>[4x]MGSTGNAEIQIIPTHSSDEEANLFAMQLASAAVLPMALKAA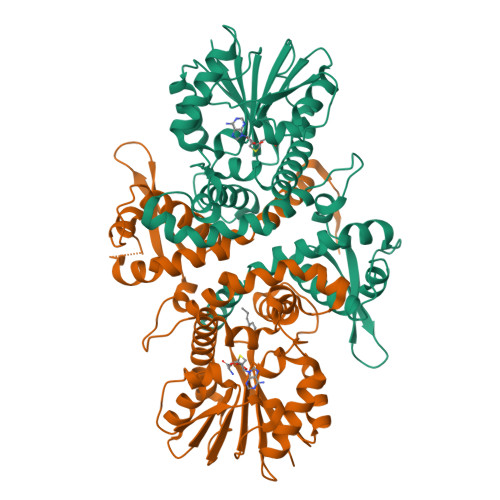IELDVLEIMAKSVPPSGYISPAEIAAQLPTTNPEAPVMLDRVLRLLASYSVVTYTLRELPSGKVERLYGLAPVCKFLTKNEDGVSLAPFLLLATDKVLLEPWFYLKDAILEGGIPFNKAYGMNIFDYHGTDHRINKVFNKGMSSNSTITMKKILEMYNGFEGLTTIVDVGGGTGAVASMIVAKYPSINAINFDLPHVIQDAPAFSGVEHLGGDMFDGVPKGDAIFIKWICHDWSDEHCLKLLKNCYAALPDHGKVIVAEYILPPSPDPSIATKVVIHTDALMLAYNPGGKERTEKEFQALAMASGFRGFKVASCAFNTYVMEFLKTA Pterostilbene | C16 H16 O3 | 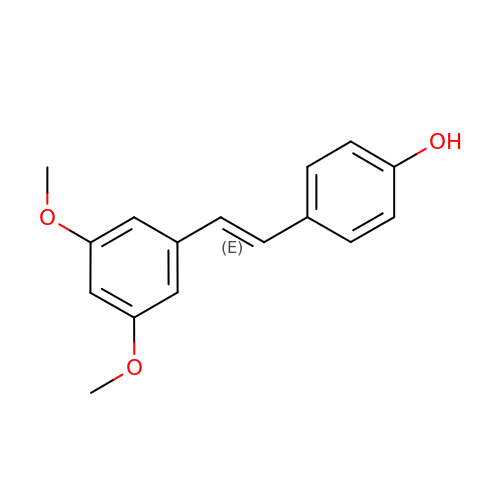VLEUZFDZJKSGMX-ONEGZZNKSA-N>DDHSELLVNTKSGKVMGTRVPVLSSHISAFLGIPFAEPPVGNMRFRRPEPKKPWSGVWNASTYPNNCQQYVDEQFPGFSGSEMWNPNREMSEDCLYLNIWVPSPRPKSTT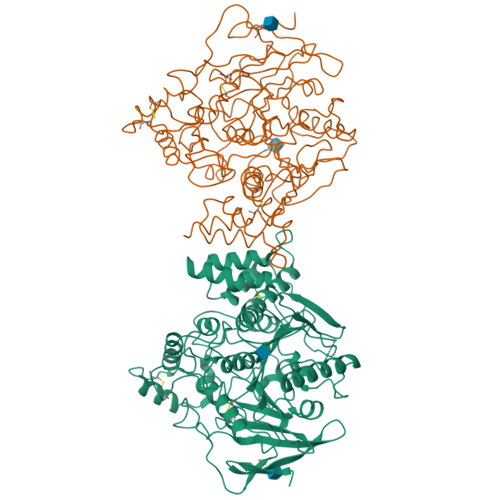VMVWIYGGGFYSGSSTLDVYNGKYLAYTEEVVLVSLSYRVGAFGFLALHGSQEAPGNVGLLDQRMALQWVHDNIQFFGGDPKTVTIFGESAGGASVGMHILSPGSRDLFRRAILQSGSPNCPWASVSVAEGRRRAVELGRNLNCNLNSDEELIHCLREKKPQELIDVEWNVLPFDSIFRFSFVPVIDGEFFPTSLESMLNSGNFKKTQILLGVNKDEGSFFLLYGAPGFSKDSESKISREDFMSGVKLSVPHANDLGLDAVTLQYTDWMDDNNGIKNRDGLDDIVGDHNVICPLMHFVNKYTKFGNGTYLYFFNHRASNLVWPEWMGVIHGYEIEFVFGLPLVKELNYTAEEEALSRRIMHYWATFAKTGNPNEPHSQESKWPLFTTKEQKFIDLNTEPMKVHQRLRVQMCVFWNQFLPKLLNATACDGELSS[2x]> MKSRTSELAVGIFVIIFGIALFFLAMKVSGLVGTNLSDGYTMKAQFDNVNGLKPRAKVTMSGV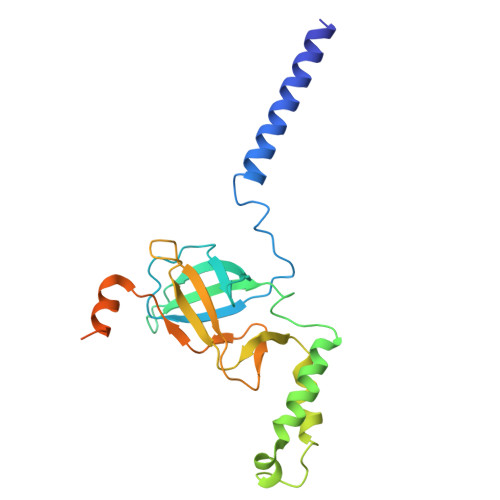TIGRVDSITLDPVTRLATVTFDLDGKLTSFNAEQLKEVQKNALDELRYSSDYTQATPAQQKTMEQQLISNMNSITSIDEDAYIMVATNGLLGEKYLKIVPGGGLNYLKRGDTISNTQGTMDLEDLISKFITGGGAGKVAAGSSSAEEKAPASTDSSAQPSFVE> MAAQRRSLLQSEQQPSWTDDLPLCHLSGVGSASNRSYSADGKGTESHPPEDSWLKFRSENNCFLYGVFNGYDGNRVTNFVAQRLSAELLLGQLNAEHAEADVRRVLLQAFDVVERSFLESIDDALAEKASLQSQLPEGVPQHQLPPQYQKILERLKTLEREISGGAMAVVAVLLNNKLYVANVGTNRALLCKSTVDGLQVTQLNVDHTTENEDELFRLSQLGLDAGK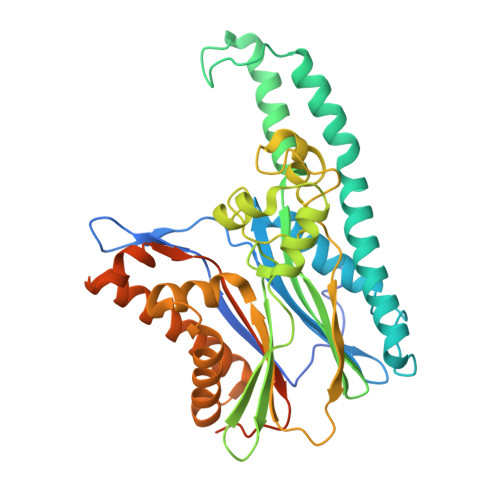IKQVGIICGQESTRRIGDYKVKYGYTDIDLLSAAKSKPIIAEPEIHGAQPLDGVTGFLVLMSEGLYKALEAAHGPGQANQEIAAMIDTEFAKQTSLDAVAQAVVDRVKRIHSDTFASGGERARFCPRHEDMTLLVRNFGYPLGEMSQPTPSPAPAAGGRVYPVSVPYSSAQSTS>MNITGKGAYDTGTYANLFQRSGYREDEIKARLEQTWNDLFYGDEHTRIYYPVGDDKGYMLDTGNDDVRSAGMSYGMMMAVQMDKKHEFDRLWNYAYTYMQHTEGRYKDYFAWHCKPDGTRLSPGPAPDGEEFFAMALFFASNRWGDGPAPYDYQAQARKILHACLHQGEQGEGDPMWEPSNRLIKFIPELPFSDPSYHLPHFYELFAQYANEQDRTFWKEAAEASRAYLRTACHPVTGLSPEYANYDGTPAPVQLHGDFRHFYSDAYRVAANVALDWEWFRKDPWQVQQSNRIQAFFSDIDVSDYRRYTIEGEPFNEPALHPVGLLATNA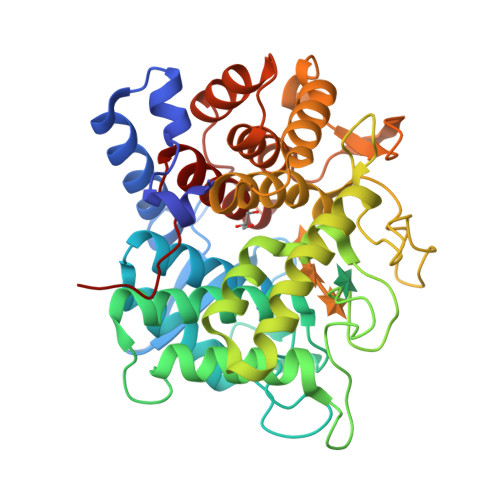MASLAADGPDADSFVKRFWNTPLRQGKRRYYDNCLYFFTMLALSGNYRVYQQAAA[2x]>MAEFRIAQDVVARENDRRASALKEDYEALGANLARRGVDIEAVTAKVEKFFVAVPSWGVGTGGTRFARFPGTGEPRGIFDKLDDCAVIQQLTRATPNVSLHIPWDKADPKELKARGDALGLGFDAMNSNTFSDAPGQAHSYKYGSLSHTNAATRAQAVEHNLECIEIGKAIGSKALTVWIGDGSNFPGQSNFTRAFERYLSAMAEIYKGLPDDWKLFSEHKMYEPAFYSTVVQDWGTNYLIAQTLGPKAQCLVDLGHHAPNTNIEMIVARLIQFGKLGGFHFNDSKYGDDDLDAGAIEPYRLFLVFNELVDAEARGVKGFHPAHMIDQFHNVTDPIESLINSANEIRRAYAQALLVDRAALSGYQEDNDALMATETLKRAYRTDVEPILAEARRRTGGAVDPVATYRASGYRA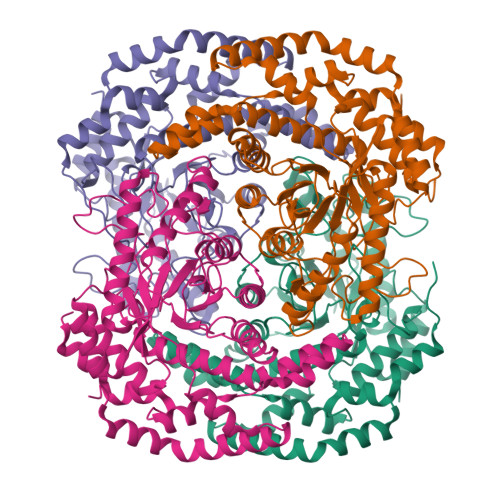RVAAERPASVAGGGGIIGSHHHHHH[4x]>[2x]PFATADIAEKMWAENYETTSPAPVLVAEGEQVTIPCTVM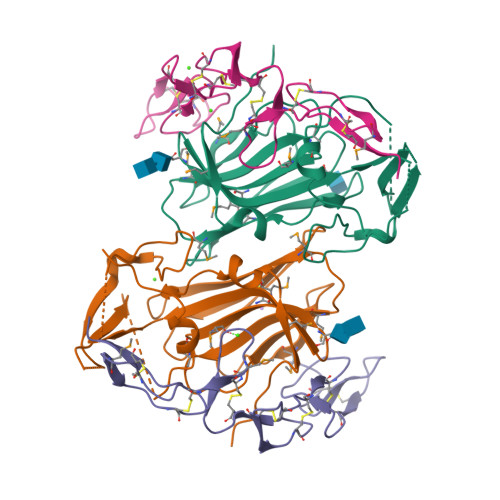THSWPMVSIRARFCRSHDGSDELILDAVKGHRLMNGLQYRLPYATWNFSQLHLGQIFSLTFNVSTDTAGMYECVLRNYSHGLIMQRFVILTQLETLSRPDEPCCTPALGRYSLGDQIWSPTPWRLRNHDCGMYRGFQRNYFYIGRADAEDCWKPACPDEEPDRCWTVIQRYRLPGD;>QQDLAPQQRAAPQQKRSSPSEGLCPPGHHISEDGRDCISCKYGQDYSTHWNDLLFCLRCTRCDSGEVELSPCTTTRNTVCQCEEGTFREEDSPEMCRKCRTGCPRGMVKVGDCTPWSDIECVHKESG[2x]>[12x]MNESAGHNIKEDYFRVDMLLNKKGQVILYGPPGTGKTWIARKYVVEETNEKTPGNKWEFITFHQSYSYEEFIEGFRPRTDNEEKIRYVVEDGIFKKIALRALVKGLFELEDATIGKDKI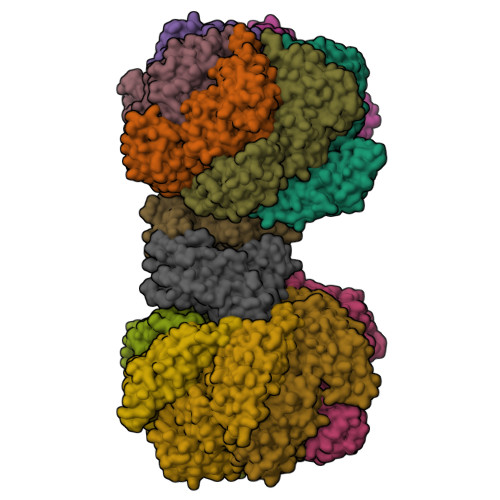HRLYILLTKKEPLSPTEYEEYLRLKRYLWELVGGLPKDKLKNLTPKFYLIIDEINRGNISKIFGELITLLEKDKRLGGENQLIVRLPYSGEPFAVPPNLYIIGTMNTADRSIALLDVALRRRFAFIEVEPRPEFLEKENLKKIREKKLKTEDRKRLNEKLNELFSKLGNDNYFLKTLLEKINVRITVVKDRDHRIGHSYFLNVETVEDLHHVWYYEVLPLLMEYFYNDWETIKWVLNEKGKEHGNVFFEKLRLTGPNGEEAYQLKVLEGDAFIGALKRIISKNTPSQEGGATTNEENSPENTQSQTEGD;>MPRLTTITLYEHDEKRYRDIAGDKKAIQDALIKLNKQFKKDFKKLDRSEDNSDTEDTIDESKGVVEVYANKIKARHYVGFAAVDNVFLQILPKVFKPKKEQTQETQEDTWEPILAFIRMLDMAYGLKIKDHDLAYLQGRNLRPNLYEVFIYLFAKSLWSEVQRGYHREYVEVHREEKFLRGKLLMSRQIRKLPHQLNTFSVEVHELIEDNLLNRIFYASVREALRRTTWGLNRKLLGELMLAFDGITPIHLRTEHFERVHFTRLNERFRRPFELAKLLFMPASGKGRSREVSGFFVDMNKLFERFIERVLVRNLPPEYKLFYQESYPFLKNQNGSSQKPDYVVRKGNTPVVVLDAKYRELKERIPSSDMLRQLYVYSRIWGYKTSHENDSKPPAVIVIPSSSTYNQGLPDKPLEFEFFDERKLFIVAYNMDYVKTGAIFKADKNFRRSLNNIIGKLNT[2x]>[4x]MAGNKKINRREEILQALAEMLESNEGASRITTAKLAKQVGVSEAALYRHFPSKTRMFEGLIEFIEESLMSRINRIFDEEKDTLNRIRLVMQL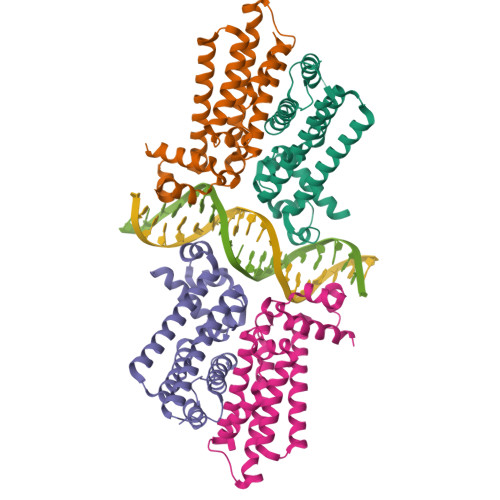LLAFAERNPGLTRILSGHALMFENERLRDRINQLFERIETSLRQILRERKLREGKSFPVDENILAAQLLGQVEGSLNRFVRSDFKYLPTANFDEYWALLSAQIK> KVFERCELARTLKRLGMDGY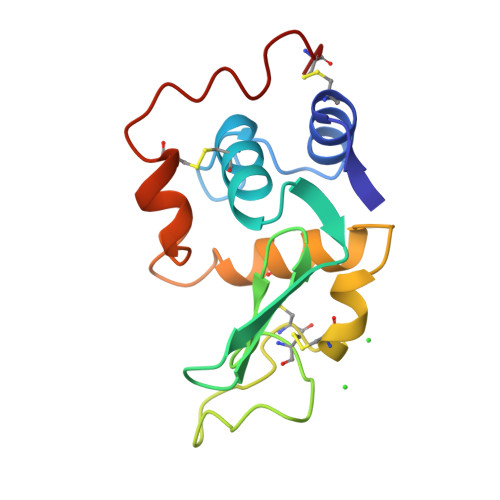RGISLANWMCLAKWESGYNTRATNYNAGDRSTDYGIFQINSRYWCNDGKTPGAVRGDSNACHLSCSALLQDNIADAVACAKRVVRDPQGIRAWVAWRNRCQNRDVRQYVQGCGV>[3x]ARMNRPAPVEVTYKNMRFLITHNPTNATLNKFIEELKKYGVTTIVRVCEATYDTTLV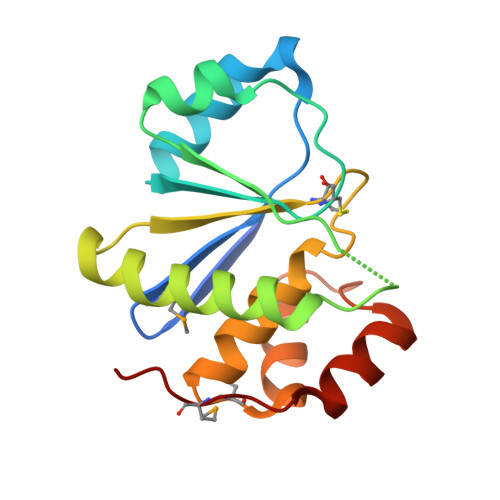EKEGIHVLDWPFDDGAPPSNQIVDDWLSLVKIKFREEPGCCIAVHCVAGLGRAPVLVALALIEGGMKYEDAVQFIRQKRRGAFNSKQLLYLEKYRPKMRLRF> RCCH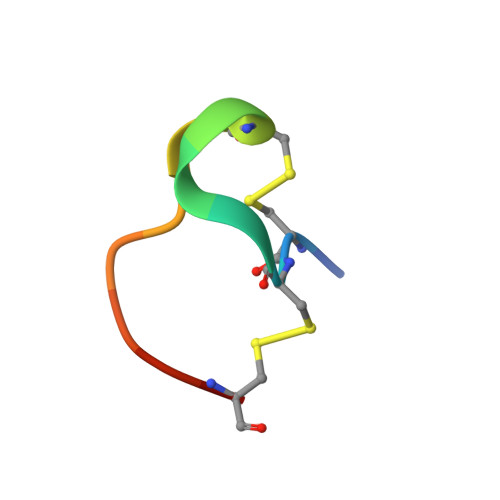PQCGMVEECR>VVCREASHAGSWYTASGPQLNAQLEGWLSQVQSTKR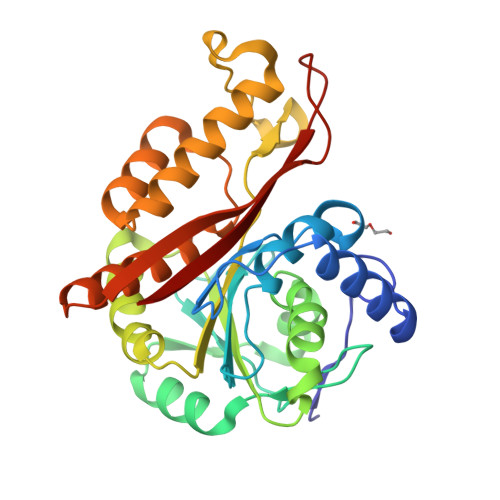PARAIIAPHAGYTYCGSCAAHAYKQVDPSITRRIFILGPSHHVPLSRCALSSVDIYRTPLYDLRIDQKIYGELWKTGMFERMSLQTDEDEHSIEMHLPYTAKAMESHKDEFTIIPVLVGALSESKEQEFGKLFSKYLADPSNLFVVSSDFCHWGQRFRYSYYDESQGEIYRSIEHLDKMGMSIIEQLDPVSFSNYLKKYHNTICGRHPIGVLLNAITELQKNGMNMSFSFLNYAQSSQCRNWQDSSVSYAAGALTVH[4x]2-(furan-3-yl)ethanoic acid | C6 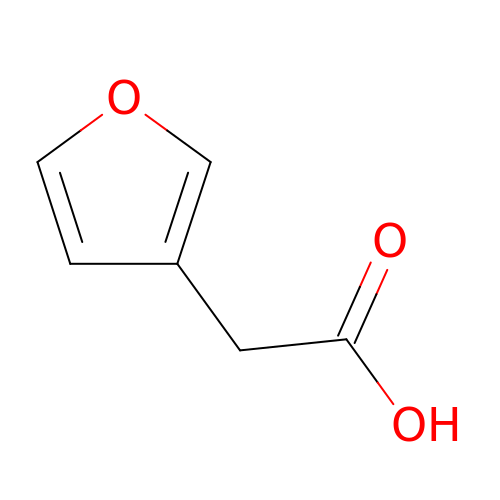H6 O3 | UUUYAVXPERPSAI-UHFFFAOYSA-N>[3x]MSNTKTASTGFAELLKDRREQVKMDHAALASLLGETP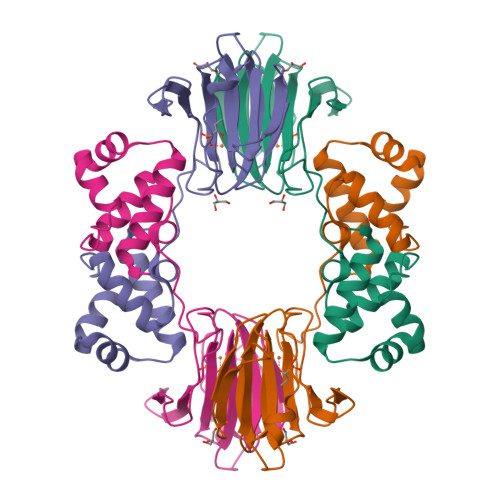ETVAAWENGEGGELTLTQLGRIAHVLGTSIGALTPPAGNDLDDGVIIQMPDERPILKGVRDNVDYYVYNCLVRTKRAPSLVPLVVDVLTDNPDDAKFNSGHAGNEFLFVLEGEIHMKWGDKENPKEALLPTGASMFVEEHVPHAFTAAKGTGSAKLIAVNF>GAQQLTPPAGTFRLGISKGTDSHWLAPQEKVKGIAFRWKALPDTRGFILEVAVTSLQQADTLFWSFGNCQPDMDINVFSVEGQAFTCYYGESMKLRTLQAVTPTDDIRLSNGRQDKTPLLLYESGKRTDRPVLAGRCPLAANSKLYF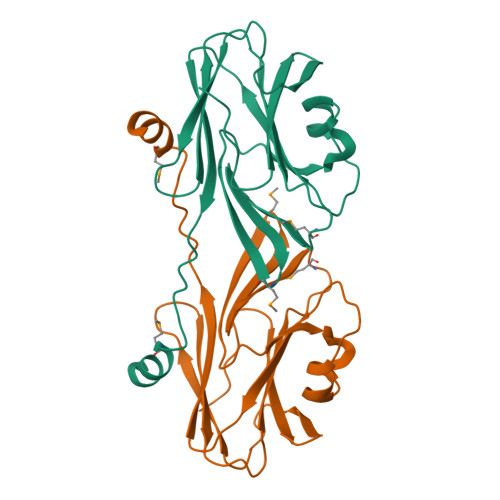CFYEQNARADYNYFMLPDLFAKIDESKHSKK[4x]>HCDLPCGVFDPAQARIEAESVKAVQEKMAGNDDPHFQTRATVIKEQRAELAKHHVSVLWSDYFKPPHFEKYPELHQLVNDTLKALSAAKGSKDPATGQ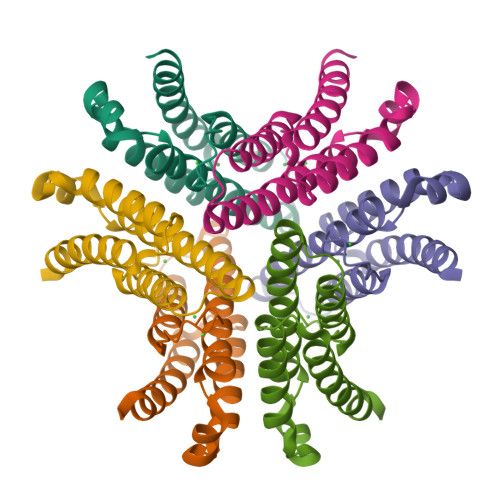KALDYIAQIDKIFWETKKA[3x]> 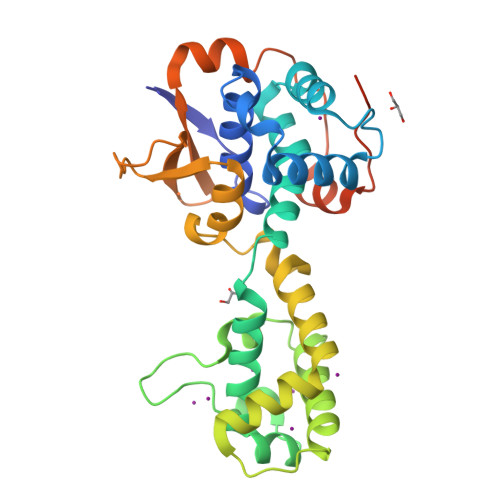GPMAKTIKATGDGACLFNAVSIGLSVEILSGRLDSQLDTPGYQALLDEFAKHHPQFNPKSWKTLKEWLAYYNDTRDIELILAPVLFNLNQKYQDHLDEEILNELTNLVWKNKANIENGQAWFQLQNTGDLGEALFPKLENLDLKKDRAPLLDKLREILKDYKLELTRENVKQFLTEKAKELLSALKKKISSDPHAFQRGYSCDELKGMTDALAISLVENREEDITDNRIKIRLENQEEHWNVLCNEEDSERFLDSTPSRLKMTSLEAYRGDKQVSAPTSEQLDLIEEPGVFLRERT>HGIRMTRISREMMKELLSVYFIMGSNNTKADPVTVVQKALKGGATLYQFREKGGDALTGEARIKFAEKAQAACREAGVPFIVNDDVELALNLKADGIHIGQEDANAKEVRAAIGDMILGVAAHTMSEVKQAEEDGADYVGLGPIYPTETKKDTRAVQGVSLIEAVRRQGISIPIVGIGGITIDNAAPVIQAGADGVSMISAISQAEDPESA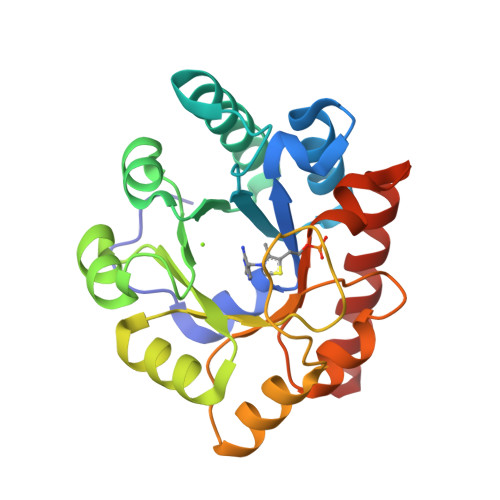ARKFREEIQTYKTGR[2x]>[2x]GSVYLRYFKGLILSDAYAPGLKWSDELKAYSALAFKYRDVRKYFLEKEIEVEENVIDSLPFPLIKDKIELRDYQAEAVKAWLKEKRGIIVLPTGAGKTQVALKIVSIMKVATLIVVPTIDLITQWKERINKYLDFDPGIIGGGEDSLKGITVITYDSAYTRAEELGNKFPLLIFDEVHHLPSEGYSIMAQLFASPYRLGLTATPERDDGKHELYPILVGPIVYRKSVEELAGKYIAKYKIKKLYVSLTNEEKKRYDGLRKKLKDFLSSRGLKLQNLDDFHRLVKLAAKDKEAREALLAWHESLNIAVNSQSKIEKL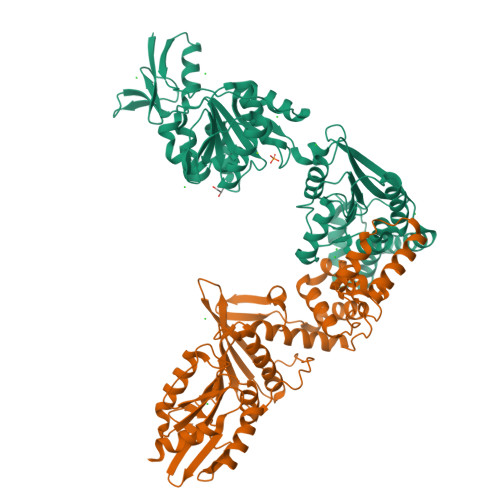REILQEYKNEKIIVFTRDTQMAYRISKTFLIPVVTYKTDKDEREEILQKFRDGEYRVIVASTVFDEGVDVPDATLAIVMGGYGTKRQFLQRLGRILRKKDKEALLIEIVTKGTADYRLSRRRRE;>[2x]MGLPWELARFSIVKDEVLPHFATNEDLDLANEIISLFKAGKKLGEIDEEIEYLEKIYDHKLVRAFVKLLTRLCEFELDSPIPPIQIRRELFKYGPVLDEKEREDIIQKVSKKLGADIMRFVFSDLDEEKKIIKAPTISAEDLIRWYNLSLLQTLLFKAYKLTVYVSSNWKEIIRRAKWLGLMYFAYDKPLRFEFLGPATLVKLTEKYGRNLAVLLQFIISSQNWKIEAELVLGKKFKRVYKLKLANFKELKELVIDEKRFDSSVEEKFYKDFTNVIKGWKIIREPEPLVVDNRVFIPDFLVEKGNLKVYVEIVGFWTKEYIKEKLDKLKKVKYPILILLNEELGKEKFNGMNVITYKRKIDISLVYKWLRELEN> MAFPELLDRVGGRGRFQLLQAVALVTPILWVTTQSMLENFSAAVPHHRCWVPLLDNSTSQASIPGDFGRDVLLAVSIPPGPDQRPHQCLRFRQPQWQLIESNTTATNWSDADTEPCEDGWVYDHSTFRSTIVTTWDLVCDSQALRPMAQSIFLAGILVGAAVCGHASDRFGRRRVLTWSYLLVSVSGTIAALMPTFPLYCLFRFLVASAVAGVMMNTASLLMEWTSAQAGPLMMTLNALG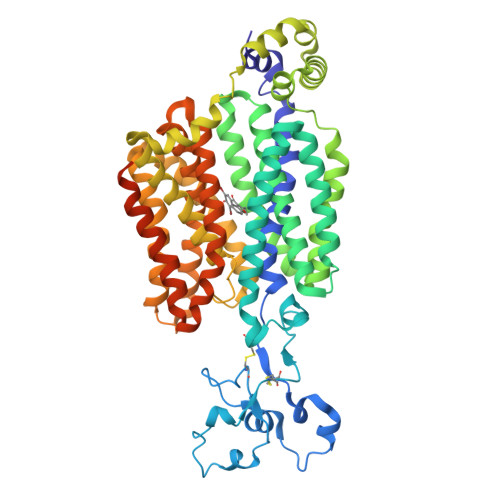FSFGQVLTGSVAYGVRSWRMLQLAVSAPFFLFFVYSWWLPESARWLITVGRLDQSLRELQRVAAVNRRKAEADTLTVEVLRSAMQEEPNGNQAGARLGTLLHTPGLRLRTFISMLCWFAFGFTFFGLALDLQALGSNIFLLQALIGIVDLPVKMGSLLLLSRLGRRLCQASSLVLPGLCILANILVPREMGILRSSLAVLGLGSLGAAFTCVTIFSSELFPTVIRMTAVGLGQVAARGGAILGPLVRLLGVYGSWLPLLVYGVVPVLSGLAALLLPETKNLPLPDTIQDIQKQSVKKVTHDIAGGSVLKSARL4-hydroxyquinoline-2-carboxylic acid | 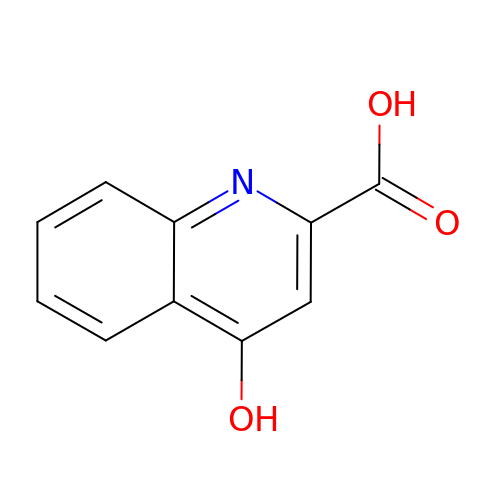C10 H7 N O3 | HCZHHEIFKROPDY-UHFFFAOYSA-N>[41x]MRINHNIAALNTLN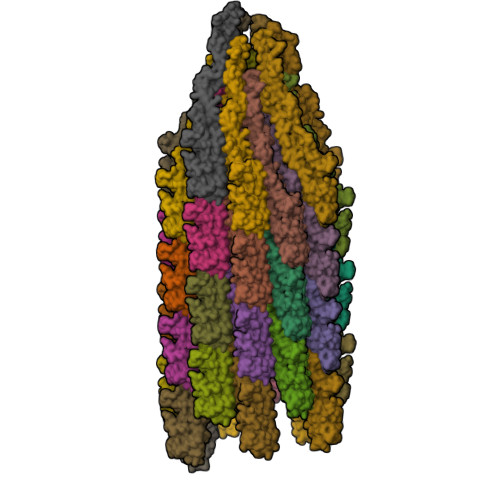RLSSNNSASQKNMEKLSSGLRINRAGDDAAGLAISEKMRGQIRGLEMASKNSQDGISLIQTAEGALTETHAILQRVRELVVQAGNTGTQDKATDLQSIQDEISALTDEIDGISNRTEFNGKKLLDGTYKVDTATPANQKNLVFQIGANATQQISVNIEDMGADALGIKEADGSIAALHSVNDLDVTKFADNAADCADIGFDAQLKVVDEAINQVSSQRAKLGAVQNRLEHTINNLSASGENLTAAESRIRDVDMAKEMSEFTKNNILSQAPQAMLAQANQQPQNVLQLLR> GSHMAGAQDFVPHTADLAELAAAAGECRGCGLYRDATQAVFGAGGRSARIMMIGEQPGDKEDLAGLPFVGPAGRLLDRALEAADIDRD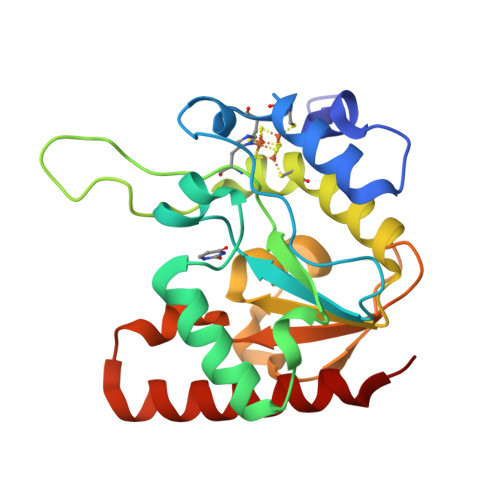ALYVTNAVKHFKFTRAAGGKRRIQKTPSRTEVVACRPWLIAEMTSVEPDVVVLLGATAAKALLGNDFRVTQHRGEVLHVDDVPGDPALVATVHPSSLLRGPKEERESAFAGLVDDLRVAADVRP RgNanOx (RUMGNA_02695) from R. gnavus ATCC 29149 catalyzes the equilibration of 2,7-anhydro-Neu5Ac and Neu5Ac. The novel oxidoreductase identified in our work showed to catalyze the conversion 2,7-anhydro-Neu5Ac to Neu5Ac in the presence of NAD+ in a reversible manner. The protein shows a Rossman fold typical of NAD-binding protein of the Gfo/Idh/MocA class characterized by a central β-sheet with helices on either side. Here, we showed that RgNanOx acts through a multistep mechanism involving a keto intermediate and cycling of NADH/NAD+.

In the RgNanOx structure, there is additional density adjacent to the nicotinamide ring that, given the high resolution of the second structure, we were able to unambiguously identify as citric acid from the crystallization buffer. Using the high-resolution structure, we used a simple modeling approach to place a molecule of DANA a transition state analog inhibitor of sialidases, in RgNanOx active site by overlapping the carboxylate acid of the DANA with each of the three carboxylate groups of citric acid. Next we manually positioned the sugar such that the H3 of the atom ring pointed toward the C4′ of the nicotinamide, as would be required for hydride transfer. These models were then minimized, and we investigated whether the H4 atom of DANA was still able to transfer to nicotinamide. Only one position where the DANA carboxylate was placed on the 2-carboxylic acid of citric remained positioned for hydride transfer. The model indicated that His-178, predicted to be a catalytic residue, is positioned to remove the proton from O4 during the oxidation step. His-176 is plausibly positioned to undertake proton transfer with the O7 of the substrate glycerol that the mechanism requires. His-175 interacts with the negatively charged carboxylic acid in the model but could play a role in proton transfer at the substrate C3 atom. Lys-93 binds to NAD+, is part of the catalytic constellation, and is also within a plausible distance for proton transfer to C3. Lys-163 binds to the NAD+ co-factor and interacts with the substrate carboxylate.

>GAMADIGSMKTVGYAIVGTGYFGAELGRIMKEQEGARIVAVLDPENGQTIAEELDCDVETDLDTLYSREDVEAVIVATPNYLHKEPVIKAAEHGVNVFCEKPIALSYQDCDEMVRTCQEHGVIFMAGHVMNFFHGVRYAKKLINDGVIGKVLYCHSARNGWEEQQPTISWKKIREKSGGHLYHHIHELDCVQFLMGGMPEEVTMTGGNVAHQGEAFGDEDDMLFVNMQFSDNRYAVLEWGSAFHWPEHYVLIQGTKGAIKIDMCDCGGTLKVDGREEHFLVHESQEEDDDRTRIYHGTEMDGAIMYGKPGKKPPMWLHSIMKNEMKYLNGILHGKEVDDEFRPLLTGEAARAAIATADACTKSRFEDRKVKLSEIIGEGSTI[2x]> MTVTRRHFLKLSAGAAVAGAFTGLGLSLAPTVARAELQKLQWAKQTTSICCYCAVGCGLIVHTAKDGQGRAVNVEGDPDHPINEGSLCPKGASIFQLGENDQRGTQPLYRAPFSDTWKPVTWDFALTEIAKRIKKTRDASFTEKNAAGDLVNRTEAIASFGSAAMDNEECWAYGNILRSLGLVYIEHQARIUHSPTVPALAESFGRGAMTNHWNDLANSDCILIMGSNAAENHPIAFKWVLRAKDKGATLIHVDPRFTRTSARCDVYAPIRSGADIPFLGGLIKYILDNKLYFTDYVREYTNASLIVGEKFSFKDGLFSGYDAANKKYDKSMWAFELDANGVPKRDPALKHPRCVINLLKKHYERYNLDKVAAITGTSKEQLQQVYKAYAATGKPDKAGTIMYAMGWTQHSVGVQNIRAMAMIQLLLGNIGVAGGGVNALRGESNVQGSTDQGLLAHIWPGYNPVPNSKAATLELYNAATPQSKDPMSVNWWQNRPKYVASYLKALYPDEEPAAAYDYLPRIDAGRKLTDYFWLNIFEKMDKGEFKGLFAWGMNPACGGANANKNRKAMGKLEWLVNVNLFENETSSFWKGPGMNPAEIGTEVFFLPCCVSIEKEGSVANSGRWMQWRYRGPKPYAETKPDGDIMLDMFKKVRELYAKEGGAYPAPIAKLNIADWEEHNEFSPTKVAKLMNGYFLKDTEVGGKQFKKGQQVPSFAFLTADGSTCSGNWLHAGSFTDAGNLMARRDKTQTPEQARIGLFPNWSFCWPVNRRILYNRASVDKTGKPWNPAKAVIEWKDGKWVGDVVDGGGDPGTKHPFIMQTHGFGALYGPGREEGPFPEHYEPLECPVSKNPFSKQLHNPVAFQIEGEKKAVCDPRYPFIGTTYRVTEHWQTGLMTRRCAWLVEAEPQIFCEISKELAKLRGIGNGDTVKVSSLRGALEAVAIVTERIRPFKIEGVDVHMVGLPWHYGWMVPKNGGDTANLLTPSAGDPNTGIPETKAFMVDVRKVWSHPQFEK;> MGKMFFVDLSRCTACRGCQIACKQWKNLPAEETRNTGSHQNPPDLSYVTLKTVRFTEKSRKGPGIDWLFFPEQCRHCVEPPCKGQADVDLEGAVVKDETTGAVLFTELTAKVDGESVRSACPYDIPRIDPVTKRLSKCDMCNDRVQNGLLPACVKTCPTGTMNFGDEQEMLALAEKRLAEVKKTYPGAVLGDPNDVRVVYLFTRDPKDFYEHAVADLAPSMMTRQQLFARLFRPRA

Metal-dependent formate dehydrogenases (Fdh) catalyze the reversible conversion of CO2 to formate, with unrivalled efficiency and selectivity. Desulfovibrio vulgaris Hildenborough (Dv) Formate Dehydrogenase 1 (DvFdhAB) is a W-containing enzyme capable of interconverting CO2 and formate under mild conditions, with high specificity and turnover rates (being especially active towards CO2 reduction, when compared with other Fdhs). DvFdhAB contains a W active site coordinated by two Molybdopterin Guanine Dinucleotides (MGD), one selenocysteine (SeCys) and one terminal sulfido ligand (=S/−SH). Additionally, four [4Fe-4S] clusters are used for electron transfer.

In this study, we soaked as-isolated crystals of DvFdhAB with sodium formate and flash cooled them in liquid nitrogen at different time points. Notably, in Fdh_1min, one formate molecule is observed for the first time close to the active site, making hydrogen bonds with Nε from R441 and Oγ from T450. Formate molecules were assigned for the first time to populate the catalytic pocket of a Fdh. One of the features in the reduction of DvFdhAB is the conformational change in MGD2 with the distortion of the ribose moiety. Here, we observed this conformational change in the first two time-points structures, whereas the remaining active site residues are in the oxidized form conformation, suggesting that the conformational change in MGD2 is the first event in the reduction process. Unexpectedly, the first noticeable change upon formate incubation was the C5′ MGD2 swing. This movement seems to be independent of the metal site reduction changes. For these residues (E443 and Q890), despite small shifts, the structures until 1.5 min are comparable to the oxidized form.>ASISARDYKDDDDKQDTFIAAVYEHAAILPNATLTPVSREEALALMNRNLDILEGAITSAADQGAHIIVTPEDAIYGWNFNRDSLYPYLEDIPDPEVNWIPCNNRNRFGQTPVQERLSCLAKNNSIYVVANIGDKKPCDTSDPQCPPDGRYQYNTDVVFDSQGKLVARYHKQNLFMGENQFNVPKEPEIVTFNTTFGSFGIFTCFDILFHDPAVTLVKDFHVDTIVFPTAWMNVLPHLSAVEFHSAWAMGMRVNFLASNIHYPSKKMTGSGIYAPNSSRAFHYDMKTEEGKLLLSQLDSHPSHSAVVNWTSYASSIEALSSGNKEFKGTVFFDEFTFVKLTGVAGNYTVCQKDLCCHLSYKMSENIPNEVYALGAFDGLHTVEGRYYLQICTLLKCKTTNLNTCGDSAETASTRFEMFSLSGTFGTQYVFPEVLLSENQLAPGEFQVSTDGRLFSLKPTSG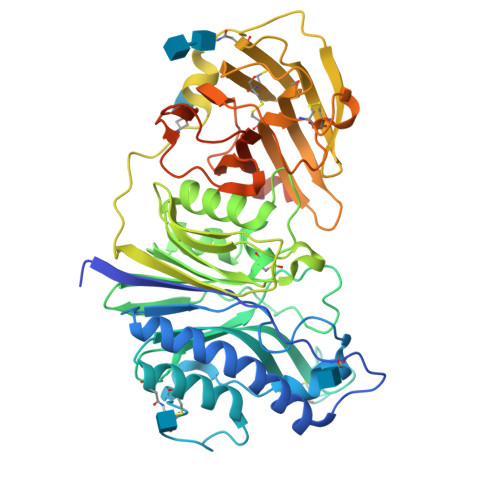PVLTVTLFGRLYEKDWASNASSGLTAQARIIMLIVIAPIVCSLSW[2x]> SPSYTVLGQLPDTDVYIDIDAYEEVKEIPGIKIFQINAPIYYANSDLYSSALKRKTGVNGSENIHTVILDFTQVNFMDSVGVKTLAGIVKEYGDVGIYVYLAGCSAQVVNDLTSNRFFENPALKELLF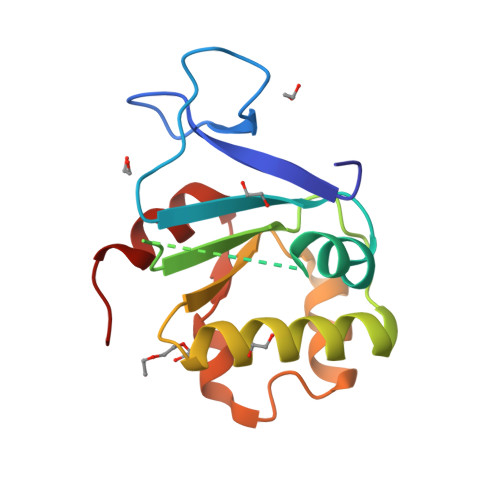HSIHDAVLGSQVREA> VEIPSSFDSRKKWPRCKSIATIRD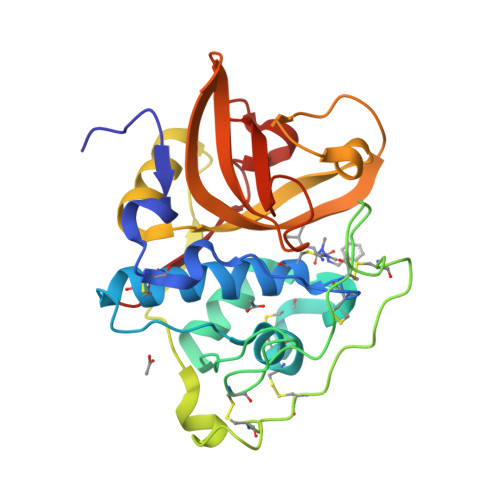QSRCGSCWAFGAVEAMSDRSCIQSGGKQNVELSAVDLLSCCESCGLGCEGGILGPAWDYWVKEGIVTGSSKENHAGCEPYPFPKCEHHTKGKYPPCGSKIYKTPRCKQTCQKKYKTPYTQDKHRGKSSYNVKNDEKAIQKEIMKYGPVEAGFTVYEDFLNYKSGIYKHITGETLGGHAIRIIGWGVENKAPYWLIANSWNEDWGENGYFRIVRGRDECSIESEVTAGRIN6-(1H-PYRAZOL-3-YL)-3-(1H-PYRAZOL-4-YL)IMIDAZO[1,2-A]PYRAZINE | C12 H9 N7 | 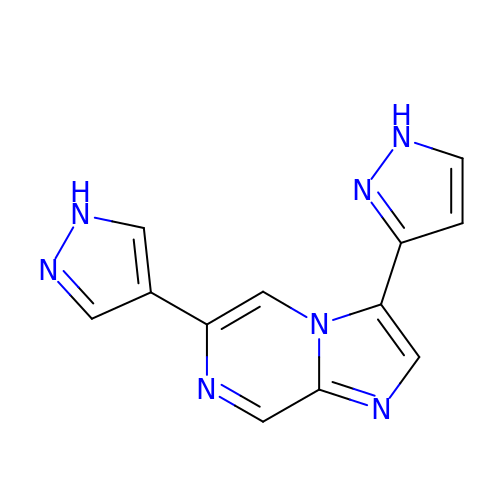ALMSMDKNGFZAEU-UHFFFAOYSA-N>EQLTKCEVFRELKDLKGYGGVSLPEWVCTTFHTSGYDTQAIVQNNDSTEYGLFQINNKIWCKDDQNPHSSNICNISCDKFLDDDLTDDIMCVKKILDKVGINYWLAHKALCSEK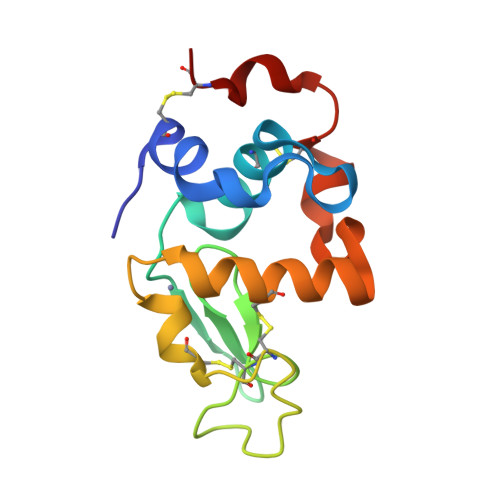LDQWLCE[6x]> KKSPQGFWQVTTKQISAAKRSGAPKRKVTTMMPVSVPKVLCRPPGQRQSEWVDLWEAYTYQKVV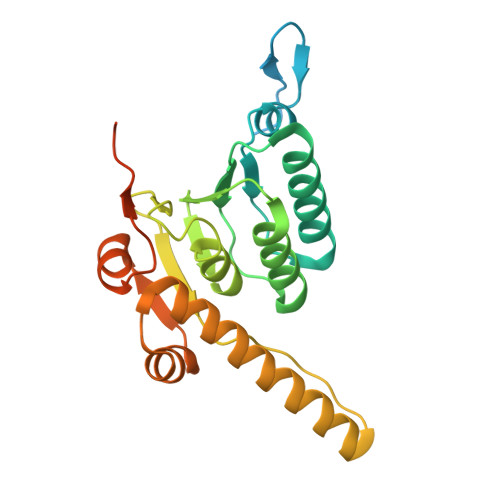FIKEAITEDVANNMIALTLYLDSLDQKRIYYWLNVPGGDVVPTLALYDTMQYVRSKTATVCYGLCLGMGGFLLTAGGEKGYRFAMPHSILMMHHPSGASRGQASEMHIESRELVRMRDYLSLLTSNATGQPYDRVIRELSRNKWMDPKQAIEYGMIDKVLTTPMPKMPSTGPSFKFERQNDELIGL>MKAPAFTEAKLQDPIPAKIYDKNGELVKTLDNGQRHEHVNLKDVPKSMKDAVLATEDNRFYEHGALDYKRLFGAIGKNLTGGFGSEGASTLTQQVVKDAFLSQHKSIGRKAQEAYLSYRLEQEYSKDDIFQVYLNKIYYSDGVTGIKAAAKYYFNKDLKDLNLAEEAYLAGLPQVPNNYNIYDHPKAAEDRKNTVLYLMHYHKRITDKQWEDAKKIDLKANLVNRTPEERQNIDTNQDSEYNSYVNFVKSELMNNKAFKDENLGNVLQSGIKIYTNMDKDVQKTLQNDVDNGSFYKNKDQQVGATILDSKTGGLVAISGGRDFKDVVNRNQATDPHPTGSSLKPFLAYGPAIENMKWATNHAIQDESSYQVDGSTFRNYDTKSHGTVSIYDALRQSFNIPALKAWQSVKQNAGNDAPKKFAAKLGLNYEGDIGPSEVLGGSASEFSPTQLASAFAAIANGGTYNNAHSIQKVVTRDGETIEYDHTSHKAMSDYTAYMLAEMLKGTFKPYGSAYGHGVSGVNMGAKTGTGTYGAETYSQYN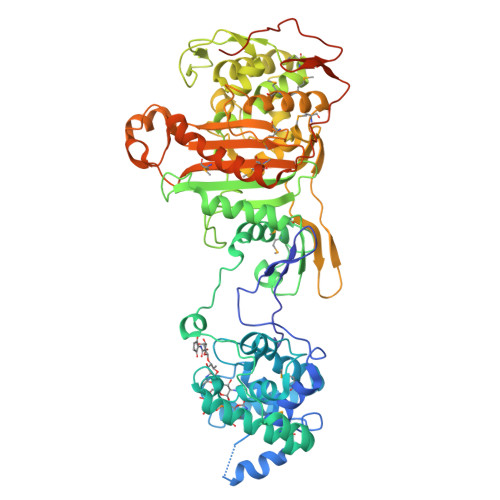LPDNAAKDVWINGFTPQYTMSVWMGFSKVKQYGENSFVGHSQQEYPQFLYENVMSKISSRDGEDFKRPSSVSGSIPSINVSGSQDNNTTNRSTHGGSDTSANSSGTAQSNNNTRSQQSRNSGGLTGIFN[2x]HuR/ELAVL1 is an RNA-binding protein involved in differentiation and stress response that acts primarily by stabilizing messenger RNA (mRNA) targets. HuR specifically recognizes adenine and uridine-rich elements (ARE) and uridine-rich sequences in 3′ untranslated regions (3′UTRs) of mRNAs. Hu/ELAV proteins share a common protein architecture with two consecutive RRMs, separated from the third RRM (RRM3) by a less conserved, flexible hinge region of variable length. Here, we report crystal structures of HuR RRM3 free and bound to U- and AU-rich RNAs.

We observed a substantial increase in RRM solubility after RNA binding and were thus able to use untagged RRM3 incubated with selected RNA ligands for structural studies of the complex. This allowed us to perform a comprehensive and comparative analysis of RRM3 interaction with three distinct RNA ligands: AUUUA motif-containing (AU6tnf), a U-rich motif with sparsely distributed adenosine residues (AU15) and a poly-U motif (U6). In the case of AU15, electron density for seven nucleotides (UUUAUUU) could be fitted. While in the structure of RRM3 with U6 and AU15, a uridine is recognized, in the case of AU6tnf RNA, an adenosine is bound in this pocket. In RRM3-AU6tnf and -AU15, the ribose in position 1 forms a (water-mediated) hydrogen bond with the main chain carbonyl of Lys285. On the 3′ end of the RNA, nucleotides in positions 5 and 6 are closer to the RRM3 β2β3 loop in case of the U6 ligand than when AU15 or AU6tnf are bound. To summarize, the core of the RNA interactions with RRM3 is formed by three binding pockets with canonical aromatic residues from RNP2 and RNP1 (Phe247, Tyr249, Phe289) that recognize a U–U–U/A RNA sequence motif. The affected area correlates best with the dimeric interface found between chains A and B in the structures of RNA-bound RRM3 suggesting this is the dimerization interface in solution. Moreover, our crystal structures of RNA-bound RRM3, together with NMR experiments indicate that the dimerization interface is formed by stacking of Trp261 and hydrogen bonds between amino acids from helix α1 and the α1–β2 loop.

>[3x]GAMGWCIFIYNLGQDADEGILWQMFGPFGAVTNVKVIRDFNTNKCKGFGFVTMTNYEEAAMAIASLNGYRLGDKILQVSFKTNKSHK> AFPDCANGPLKSNLVCNASADPVSRAKALVDALTLEELVNNTVNASPGVPRVGLPPYNWWSEALHGVARSPGANFSTVPGSPFSSATSFPQPIILGATFDDDLIHSIATVISTEARAFNNAGRAGLDFFTPNINPFKDPRWGRGQETPGEDPYHIAQYVYQLITGLQGGLSPDPYYKVVADCKHFAGYDLEDWHGNNRMAFNAVISTQDLAEFYTPSFQSCVRDAHVGSVMCSYNAVNGVPSCASPYLLQDLIRDHFGLGDGWITSDCDAVDNVFDPHNYTSTLVNASAVSLKAGTDVDCGTTYSQTLVDAVNQKLVTEDDVKTSMVRLYSSLVRLGYFDSPENQPWRQLGWADVNTPSAQALALTAAEEGVVLLKNDGTLPLSRRIKHIAVVGPWANATTQMQGNYQGIAPFLISPLQALQDAGFHVSFANGTAINSTDTSGFASALMAAKAADAIVFAGGIDETIESEGHDRDSIEWPGNQLDLIEQLAALRKPLIVLQMGGGQVDSSSLKASKAVNALLWGGYPGQSGGTAIVNILTGKTAPSGRLPITQYPAAYVDAIPMTDMALRPSSSSPGRTYKWYTGTPVFDFGFGLHYTSFKLSWAASPPSRFDISSLVAGAKHAGVAFTDLAPLFTFHVAVKNSGKVTSDYVALLFAHTTVGPSPAPQQELVAYTRVKGITPGRTATAALSVTLGSIARVDESGVRSLYPGKYSVWVDTTREIMHTFELTGKTTQILGWPQPR

Here, to gain a better understanding of fungal xylan degradation systems, which can enhance enzymatic saccharification of plant cell walls in industrial processes, we conducted a comparative study of two glycoside hydrolase family 3 (GH3) β-xylosidases (Bxls), one from the basidiomycete Phanerochaete chrysosporium (PcBxl3), and the other from the ascomycete Trichoderma reesei (TrXyl3A). The xylan main chain is degraded into xylooligosaccharides with low DPs by xylanase, and these products are further degraded into xylose by β-xylosidases (Bxls). PcBxl3 consists of three domains: (β/α)8 domain, (α/β)6-sandwich domain, and fibronectin III (FnIII)-like domain. The relationship between substrate specificity and degree of polymerization of substrates suggested that PcBxl3 preferentially degrades xylobiose (X2), while TrXyl3A degrades longer xylooligosaccharides.

To uncover the structural differences between PcBxl3 and TrXyl3A, the crystal structures of both enzymes were solved. There is a single molecule of PcBxl3 in the asymmetric unit, whereas there is a protein dimer in the case of TrXyl3A. N-Acetylglucosamine moieties were found at Asn17, Asn40, Asn74, Asn279, Asn286, Asn398, Asn432, and Asn437 of free PcBxl3. The overall structure and order of these domains are the same as those of TrXyl3A. The FnIII-like domain is connected to the active domain by a linker, as in other GH3 enzymes. The conformation of Glu470 (PcBxl3) is the same in the native and liganded structures of PcBxl3, but Glu492 (TrXyl3A) has different conformations in native and liganded TrXyl3A.> MAHHHHH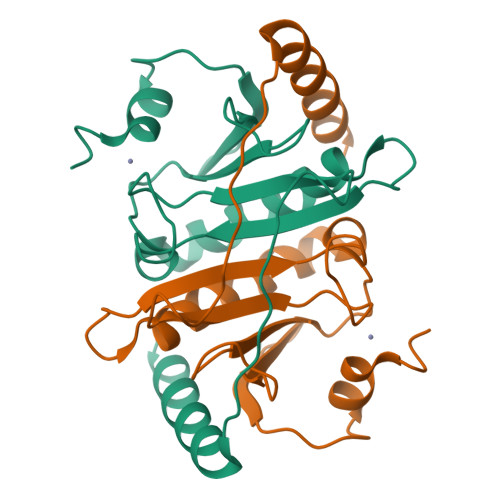HMAANCIFCKIIKGDIPCAKVAETSKALAFMDINPLSRGHMLVIPKEHASCLHELGMEDAADVGVLLAKASRAVAGPDGSMQYNVLQNNGSLAHQEVPHVHFHIIPKTDEKTGLKIGWDTVKVASDELAEDAKRYSEAIAKI Previous studies indicated that the small protein LpdD (lp_0272) is associated with the UbiD-type gallate decarboxylase LpdC (lp_2945) in Lactobacillus plantarum. The crystal structure of the purified LpdD reveals a dimeric protein with structural similarity to the eukaryotic heterodimeric proteasome assembly chaperone Pba3/4. Solution studies demonstrate that LpdD protein specifically binds to reduced prFMN species only. The addition of the LpdD–prFMNH2 complex supports reconstitution and activation of the purified E. coli apo-UbiD in vitro, leading to modest 3,4-dihydroxybenzoic acid decarboxylation. These observations suggest that LpdD acts as a prFMNH2-binding chaperone, enabling apo-UbiD activation through enhanced prFMNH2 incorporation and subsequent oxidative maturation.

Given both H35 and H61 are strictly conserved, we made LpdD H35A and H61A variants to test for the effect of an intact metal-binding site on prFMNH2 binding. The H61A variant crystallized in the same space group and conditions as the WT LpdD, and superposed with the Mn2+-bound WT LpdD monomer (0.24 Å rmsd). The loop region spanning residues 55 to 62 was disordered for both monomers in the AU. Residual electron density was present located next to H35 and D63 that was assigned to a weakly bound Mn2+. When tested using whole-cell decarboxylation assays, both variants displayed reduced activity when compared with WT LpdD whole-cell assays, with H35A more affected than H61A. In vitro reconstitution of the purified H61A variant reveals this mutation does not abolish prFMNH2 binding, whereas the purified H35A variant did not bind prFMNH2 under the conditions used. This suggests that His35—and by extension metal binding—is more important for LpdD function in vivo compared with H61, although neither are essential under the conditions tested. While mutagenesis of either H35 or H61 affects metal binding and, in the case of H35, prFMNH2 binding in vitro, both variants retain residual activity when assayed in E. coli whole-cell context.

>[2x]AAMATFTTEQAGYQMQAILQVIGYDLLIVVTGGTNPHIGDVTTLTASTVPETVKFPSHDGRFHKDNFISERMAKRIQRYLAGSCTITAGIHVNQITKAQIAAAAPMTDDLSRQIISWLQAHPVQAEKPEYYGQDEQPR>GAMDPFMSPERRPADIRRATEADMPAVCTIVNHYIETSTVNFR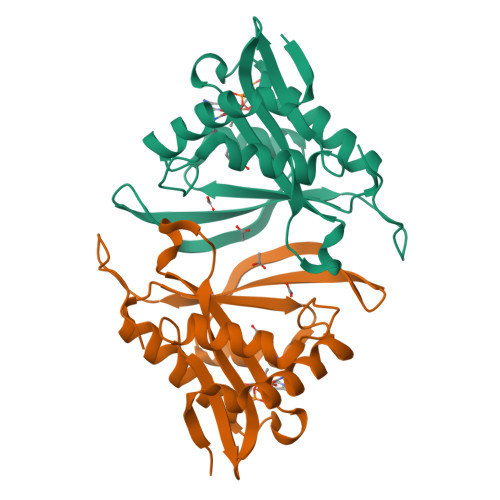TEPQEPQEWTDDLVRLRERYPWLVAEVDGEVAGIAYAGPWKARNAYDWTAESTVYVSPRHQRTGLGSTLYTHLLKSLEAQGFKSVVAVIGLPNDPSVRMHEALGYAPRGMLRAAGFKHGNWHDVGFWQLDFSLPVPPRPVLPVTEI[4x]> GLNSVIKPTKYKPVPDEEPNSTDVEETLKRIQNNDPDLEEVNLNNIMNIPVPTLKACAEALKTNTYVKKFSIVGTRSNDPVAFALAEMLKVNNTLKSLNVESNFISGSGILALVEALQSNTSLIEL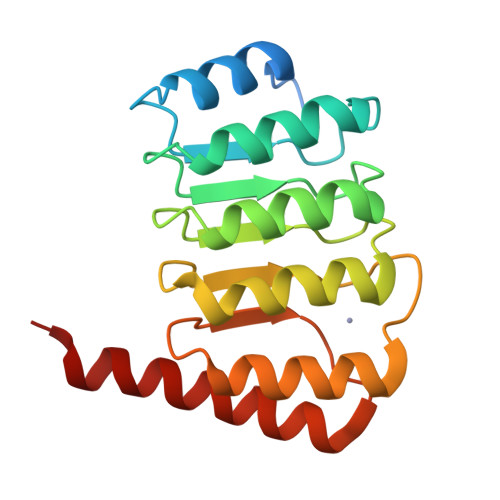RIDNQSQPLGNNVEMEIANMLEKNTTLLKFGYHFTQQGPRLRASNAMMNNNDLVRKRRL>[4x]AFTCH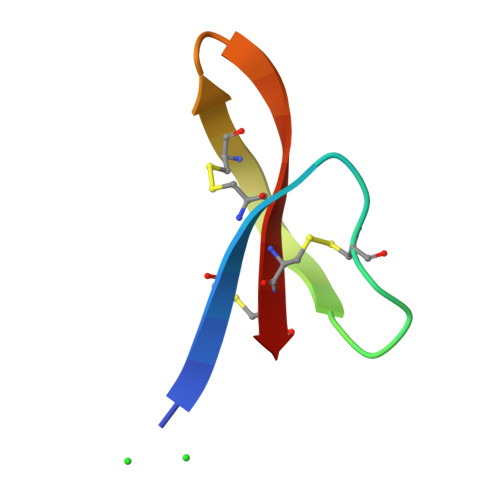CRRSCYSTEYSYGTCTVMGINHRFCCL>[2x]GENGESVVVLDKYGYPILYAPEEIGEEKEYSKYEDVVIEWNPSVTPVQIEKNYEVKFDVRQVKLRPPKVKNGSGKEGEIIVEAYASLFKSRLSKLKRILRENPEISNVVDIGKLNYVSGDEEVTIIGLVNSKRETNRGLIFEVEDKTGIVKVFLPKDSEDYREAFKVLPDAVVAFKGFYSKKGIFFANKFYLPDVPLYRKQKPPLEEKVYAILISDIHVGSREFCEKAFLKFLEWLNGHVESKEEEEIVSRVKYLIIAGDVVDGIGIYPGQYSDLVIPDIFDQYEALANLLANVPEHITMFIGPGNHDAARPAIPQPEFYKEYAKPIYKLKNAIIISNPAVIRLHGRDFLIAHGRGIEDVVSFVPGLTHHKPGLPMVELLKMRHLAPTFGGKVPIAPDPEDLLVIEEVPDLVQMGHVHVYDAVVYRGVQLVNSATWQAQTEFQKMVNIVPTPAKVPVVDVESARVVKVLDFSGWC

PolD exists in all Archaea, except Crenarchaea, and is a replicative polymerase responsible for initiating DNA synthesis at both leading and lagging strands5678. It is composed of a large catalytic subunit (DP2) and a smaller subunit with 3′–5′ proofreading exonuclease activity (DP1)5. To help resolve the uncertainty concerning the evolutionary origins of D-family DNAP, we determined the crystal structures of two large fragments of both DP1 and DP2 subunits of the Pyrococcus abyssi PolD. While the interaction between the two subunits is essential for the full activity of PolD71413, both DP1 and DP2 constructs described here are capable of digesting mispaired 3′–5′ nucleotides and of extending a DNA primer in a templated manner, respectively. Both DP1 and DP2 crystal structures were determined individually by experimental phasing and refined at final resolutions of 2.5 and 2.2 Å, respectively.

The structure of DP1 presented here encompasses amino acids 144–622, leaving out a flexible N-terminal region that is not evolutionary conserved and not needed for exonuclease activity. DP1 structure shows an insertion of an oligonucleotide/oligosaccharide binding (OB) domain in the N-terminal region of the large calcineurin-like phosphodiesterase (PDE) domain. The PDE domain contains five conserved phosphodiesterase motifs, which form the nuclease active site. Metal ions are tetrahedrally coordinated by seven conserved residues distributed in several phosphodiesterase motifs (D363, H365, D407, N453, H500, H563 and H565). To gain insight into the catalytic exonuclease mechanism of PolD, DP1 was co-crystallized together with deoxy-adenosine monophosphate (dAMP) that mimics the 3′-end of the DNA being digested. In contrast to Mre11, the adenine base binds into a narrow groove of the DP1 active site, contributed by the β8–α5 loop and α-helix α9 from one side, and the α8–β13 loop and α-helix α7 from the other side. The adenine base mainly binds through hydrophobic interactions with the side chains of Y415, V593, F589 and the alkyl moiety of K536. As expected for a non-selective nuclease, these residues do not show specific interactions with the adenine base, but instead define a pocket that partially masks the Watson–Crick face of the bound nucleotide. This observation provides a structural rationale to biochemical assays showing that DP1 exonuclease prefers mispaired nucleotides over paired nucleotides24.Condensin protein complexes coordinate the formation of mitotic chromosomes and thereby ensure the successful segregation of replicated genomes. Here, we identify a direct DNA-binding site in the eukaryotic condensin complex, which is formed by its Ycg1Cnd3 HEAT-repeat and Brn1Cnd2 kleisin subunits. A peptide loop of the kleisin subunit encircles the bound DNA and, like a safety belt, prevents its dissociation. Firm closure of the kleisin loop around DNA is essential for the association of condensin complexes with chromosomes and their DNA-stimulated ATPase activity.

To gain detailed insight into the nature of the DNA binding site, we solved crystal structures of the Ycg1–Brn1 subcomplex of Saccharomyces cerevisiae (Sc) and of the homologous Cnd3–Cnd2 subcomplex of Schizosaccharomyces pombe (Sp) to 2.8 Å and 2.6 Å resolution, respectively. Both structures are strikingly similar and reveal a harp-shaped conformation of the HEAT-repeat subunit, with the kleisin subunit winding along the concave surface of the HEAT-repeat solenoid. The peculiar curvature of Ycg1 and Cnd3 has its cause in three discontinuities in the directionality of the solenoid formed by the 19 HEAT-repeat motifs. One of the two molecules in the asymmetric unit of the Ycg1–Brn1 and Cnd3–Cnd2 crystals shows additional electron density for a segment that corresponds to a long helix (α1) in the N-terminal region of the kleisin subunit. This helix and the succeeding well-ordered turn stack onto HEAT motifs 16 and 17 and onto the α4 segment of the kleisin via several highly conserved aromatic residues in a manner that resembles a “latch” that has been inserted into a “buckle”. Through the interaction of latch and buckle regions, the kleisin subunit adopts a loop configuration. The absence of density for the latch segment in half of the complexes suggests that the α2 to α4 segments of the kleisin subunit are sufficient for complex formation with the HEAT-repeat subunit.

>[2x]MSCIQIISSSQTSIAGHRKLCNKLFTLRTQEGFETDILRALNIILTVKKGNSNADRVLRFLVTFVNYLQQKDPEIDIVQPILKHILRGLDAKDKTVRYRCCQIIARVVNCVKEIDDDLYNTLKEKLLSRVLDRESIVRLEAVVALSRLQEDTGDEENDVRNILLFLLQNDPSSEVRRSVLLNIEVSNSTLPFILERARDVDAANRKCVYARVLPKIGDFRYLSIKKRVRILKWGLNDRDESVEKAAADMLAYQWIENADNNLLELLERLDVSNNSDVAVLAIKKFFDVRVDSLSQLEFPEQFWLELTAESSLLARTFNEICIEKNYTDLLDKMPEVVQLTYYIERQYVSLRDKSSYDESCFIIEQLLYIGLSQDMVDEIGRRKLLKSLTNSLSTMALPDSLISLHIELLRKLCSSENDFCSLLVEIITEVFEQGHSQNPNELNEPEPDDMDGYKEAFNELRCLSYVQCLFENITSSLNENLYMVDMLKTLIIPAVRSHDLPIREKGLECLSLVCLLNADLAFENVPLYLHCYEKGSVVLKCTAIRTLTDMLIQHGKAKFTEYEDAISSILFEALGEFENAELQTLGAEAIAKLLVILHYRDELFLKPLIIQYFEPNTVDNHALRQVLGYFFPVYAFGAHENQWRIATIFCDALLSLLEIYRDLDEDDVQLSIGHIAQQMLDWTDNEKLYERKTQTGDDYIALNHNVHLHLANMIFESLPNASEGKERKFMISLLGKLKIPTDLPSSDYQRTKRKLETYESHGFTMDSTSLSILAKFERMLLQNEEARS;>GPLGHMNGVYEYFDKSMKKNWAGPEHWRIQALRKNINNASTVFNSSNTAESSDNVSRSLSSTERKKRRELDNAIDFLQEVDVEALFTPATSSLKLPKSHWKRHNRCLLPDDYQYDSKRLLQLFLKPKMSVLPNAD[2x]> VDCSEYPKPACTLEYRPLC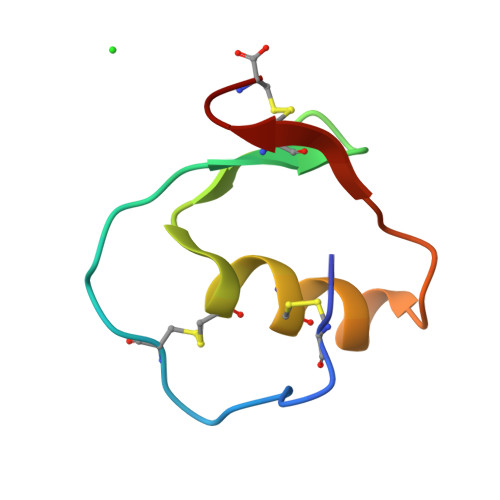GSDNKTYGNKCNFCNAVVESNGTLTLSHFGKC>[2x]MRYPEHADPVITLTAGPVNAYPEVLRGLGRTVLYDYDPAFQLLYEKVVDKAQKAMRLSNKPVILHGEPVLGLEAAAASLISPDDVVLNLASGVYGKGFGYWAKRYSPHLLEIEVPYNEAIDPQAVADMLKAHPEITVVSVCHHDTPSGTINPIDAIGALVSAHGAYL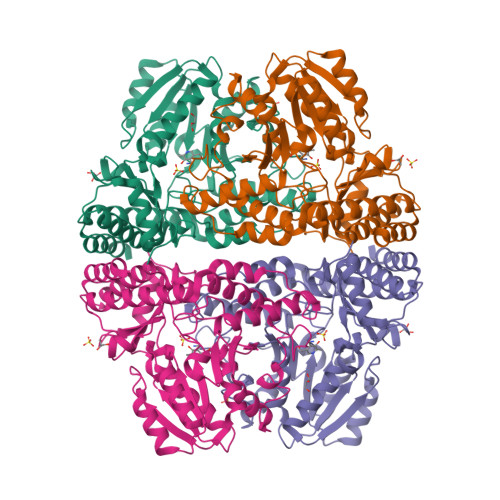IVDAVSSFGGMKTHPEDCKADIYVTGPNKCLGAPPGLTMMGVSERAWAKMKANPLAPRASMLSIVDWENAWSRDKPFPFTPSVSEINGLDVALDLYLNEGPEAVWARHALTAKAMRAGVTAMGLSVWAASDSIASPTTTAVRTPDGVDEKALRQAARARYGVVFSSGRGETLGKLTRIGHMGPTAQPIYAIAALTALGGAMNAAGRKLAIGKGIEAALAVIDADA>[4x]MGSSHHHHHHSSGLVPRGSHMPATHHSSATSAERPTVVGRIPVLDVRPVVQRGRRPAKAVTGESFEVSATVFREGHDAVGANVVLRDPRGRPGPWTPMRELAPGTDRWGATVTAGETGTWSYTVEAWGD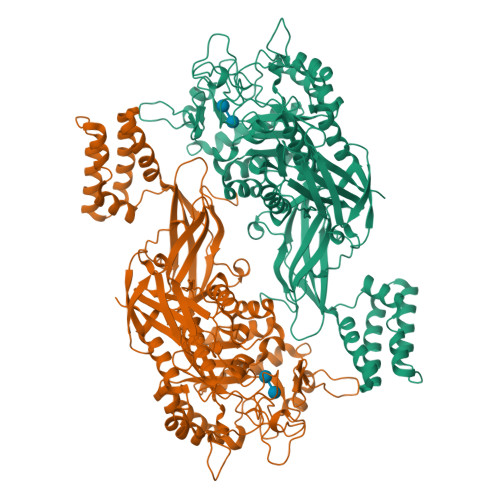PVTTWRHHARIKIPAGLDTDLVLEEGARLYERAAADVPGREDRRELLAAVDALRDESRPAASRLAAALTPQVDAVLARHPLRDLVTSSDPLPLLVERERALYGAWYEFFPRSEGTPHTPHGTFRTAARRLPAIAAMGFDVVYLPPIHPIGTTHRKGRNNTLSATGDDVGVPWAIGSPEGGHDSIHPALGTLDDFDHFVTEAGKLGLEIALDFALQCSPDHPWVHKHPEWFHHRPDGTIAHAENPPKKYQDIYPIAFDADPDGLATETVRILRHWMDHGVRIFRVDNPHTKPVAFWERVIADINGTDPDVIFLAEAFTRPAMMATLAQIGFQQSYTYFTWRNTKQELTEYLTELSGEAASYMRPNFFANTPDILHAYLQHGGRPAFEVRAVLAATLSPTWGIYSGYELCENTPLREGSEEYLDSEKYQLKPRDWTRAAREGTTIAPLVTRLNTIRRENPALRQLRDLHFHPTDKEEVIAYSKRQGSNTVLVVVNLDPRHTQEATVSLDMPQLGLDWHESVPVRDELTGETYHWGRANYVRLEPGRTPAHVCTVLRPSHPQIGGSHTT>MLAKRIDAALILKDGRVVKGSNFENLRDSGDPVELGKFYSEIGIDELSFWDITASVEKRKTMLELVEKVAEQIDIPITVGGGIYDFETASELILRGADKVEINTAAVENPSLITQIAQTFGSQAVVVYIAAKRVDGEFMVFTYSGTKNTGILLRDWV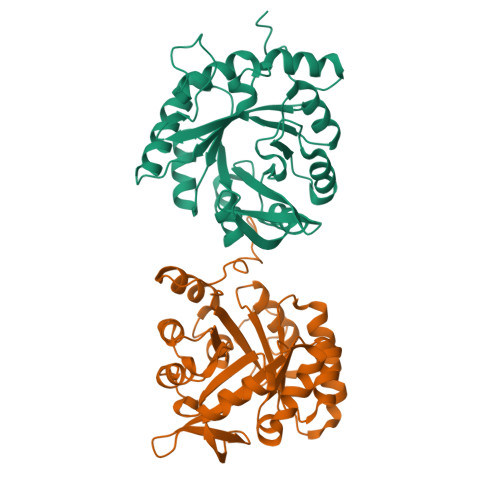VEVEKRGAGEIVLGSIDRLGTKSGYDTEMIRFVRPLTTLPIIAHRGAGKTEHFLEAFLAGADAAKADSVFHSREIDVRELKEYLKKHGVNVRLEGLGSLEHHHHHH[2x]> ANGPELIIEDTGLCTSFMLLDNIPSAHLTKELIGFTWFMQMYQMTPPLPEGAVNRIVCMTNWASLGDEGRGLEVRLPPPTDSSVHAYKTVLSRGYIDNAQFNPLALRSNVLLMLLQFTLSNLKINKSSTFTSDVTTITSGRMIRAFEGRPELLALAYPGRAVLPTQTKNAQFLSTAIADRIGRLDRANLIGGEVSAMVECMELCDALTLHIRETYIMLLRSMHQDPTQIVQIVNECANNLLNSTIPISLRPTILCPWFASSEDLRLQEVMHLVNISSNTAAALPLVEALSTLLRSVTPLVLDPTVLTNAITTISESTTQTISPISEILRLLQPMGNDYAAFWKCIASWAYNGLVTTVLSEDAFPDSSQSITHLPSMWKCLFLTLAGPMTSDPHSPVKVFMALANLLAQPEPIAIGVPGMHQTTPASQFSHPGVWPPGFLNPQLINPQQAPLLRAFAEHIRANWPQPSEFGYGSTLQGSANLFIPSNRMVYPWPNQPLPRLTVAPTYDSAMSNWISTTIAFFIRVVNSVNMTATVNDLTRRTMTGVMTAMRQVKTMTPFYIQHMCPTELSVLASVTVTPPFQVPFTRLVQNDVITNVLVARVDPAQRGDAAVDIRATHATFAAALPVDPAAIVVAMLCGQTETNLIPSHHYGKAFAPLFASNAMFTRNQRAVITREAFVCARSAVAQCQDAGFLVPRPLDALRQFDVTSAAAAEIMHAVNDAFKTAFDLDGALLDGLALYGDPRIADLSAAYLQYGGNVVREHVPPGPSHIHRALQQVESTFMAEMNLFNVARGNLYLVQTATNGNWSPMAPVAAPPFVRGGPNVRVVGR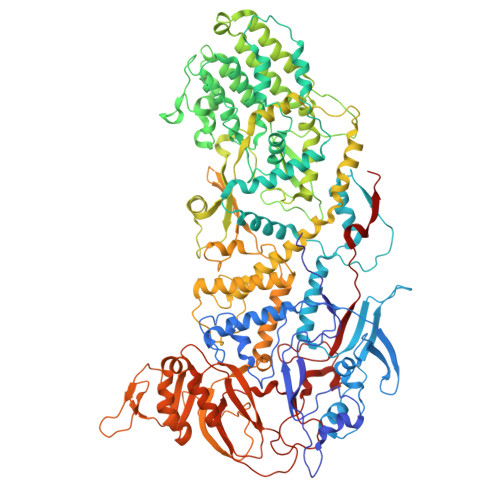FGTIVPRPNGLEPQLIDDGNVPRDIAGDWVYPSDVLQVSVAVFRDYVWPMVKAGRTRVLVELGHYVYTLHYYDPQISLDEAPILEEWLSKINPAGIPPVPFCIPIPQVYPCITARRVHYAFTSENNNDSLFSTNAASIDTAFGENAAVSPLRWPGLVDPNYRVGTNDLPNRITLYNSLYRYNFTYPTLDGIMYVRSAT> MAYKRSQILICGGTGCTSSGSMVLVKELKKELVKHDILDEVEVVTTGCFGLCELGPVVIVYPEGTFYSRVEAADIPEMVEEHLVKGRPLDRLIYNEKGDGHHPLSINELGFFKKQRRIALANCGVINPENIDEYIGFDGYLALEKVLLTMSPVDVINEVKASGLRGRGGGGFPTGLKWQFAHDAVSEDGIKYVACNADEGDPGAFMDRSVLEGDPHAVIEAMAIAGYAVGASKGYVYVRAEYPIAVNRLQIAIDQAKEYGILGENIFETDFSFDLEIRLGAGAFVCGEETALMNSIEGKRGEPRPRPPFPANKGLFGKPTVLNNVETYANIPKIILNGAEWFASVGTEKSKGTKVFALGGKINNTGLLEIPMGTTLREIIYEIGGGIPNGKAFKAAQTGGPSGGCLPESLLDTEIDYDNLIAAGSMMGSGGLIVMDEDNCMVDVARFFLDFTQDESCGKCPPCRIGTKRMLEILERICDGKG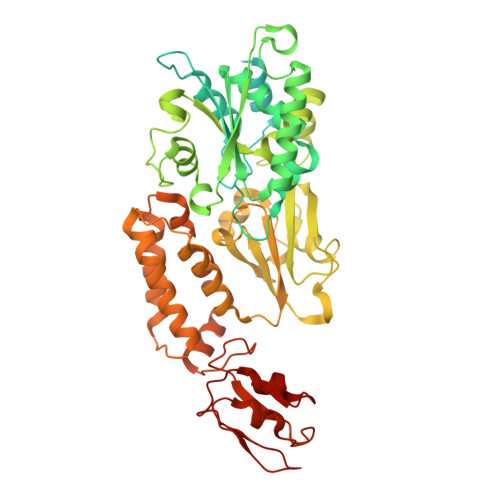VEGDIERLEELAVGIKSSALCGLGQTAPNPVLSTIRFFRDEYEAHIRDKKCPAGVCKHLLDFKINADTCKGCGICAKKCPADAISGEKKKPYNIDTSKCIKCGACIEACPFGSISKA>[2x]GAMGMTTDEGAKNNEESPTATVAEQGEDITSK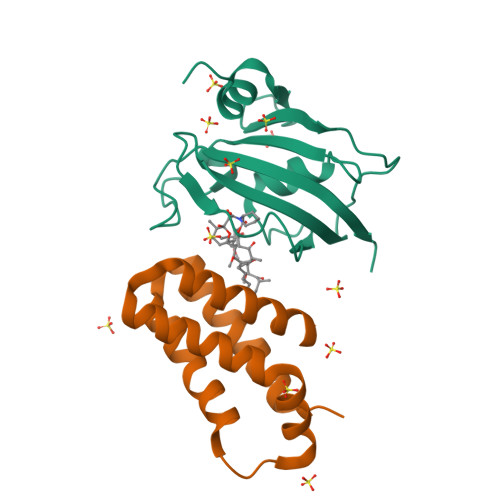KDRGVLKIVKRVGNGEETPMIGDKVYVHYKGKLSNGKKFDSSHDRNEPFVFSLGKGQVIKAWDIGVATMKKGEICHLLCKPEYAYGSAGSLPKIPSNATLFFEIELLDFKGE;>GAMDPEFMEMWHEGLEEASRLYFGERNVKGMFEVLEPLHAMMERGPQTLKETSFNQAYGRDLMEAQEWCRKYMKSGNVKDLTQAWDLYYHVFRRISKQ[2x]> ADDAKPRVKVPSSAKA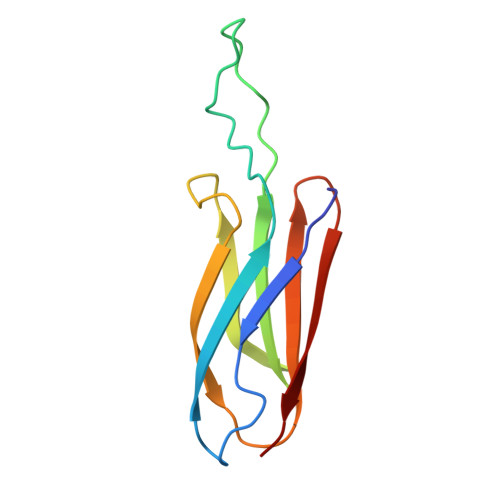GETVTVKALISHKMESGQRKDADGKLIPRSIINRFTCELNGVNVVDVAIDPAVSTNPYFEFDAKVDAAGEFKFTWYDDDGSVYEDVKPIAV>[2x]APDWVPPEVFDLVAEDKARCMSEHGTTQAQIDDVDKGNLVNEPSITCY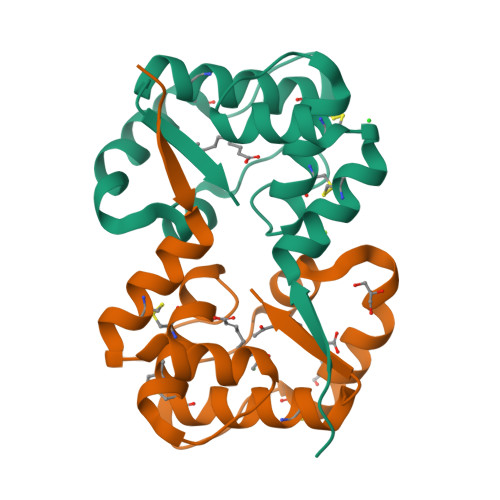MYCLLEAFSLVDDEANVDEDIMLGLLPDQLQERAQSVMGKCLPTSGSDNCNKIYNLAKCVQESAPDVWFVI Fungal immunomodulatory proteins (FIPs) are a group of low-molecular-weight (MW) proteins investigated as potential anti-tumor drugs. FIP-nha (from Nectria haematococca) contains two glycosylation sites at positions N5 and N39. In this study, the impact of glycosylation on the bioactivity and biochemical characteristics of FIP-nha (from Nectria haematococca) is described. Taken together, these findings indicate that glycosylation of FIP-nha impacts its thermostability and digestion resistance.

To study the impact of glycosylation on functionality of rFIP-nha, two single mutants (N5A and N39A) and one double mutant (N5+39A) were constructed to remove glycosylation sites. The SDS-PAGE results showed that the purified WT, N5A and N39A were partially glycosylated, while the N5+39A variant was indeed unglycosylated. However, we only managed to obtain crystals and solved the structures of WT, N39A and N5+39A. Unfortunately, none of the structures contained a density indicative of N-glycosylation. SLS and native-PAGE results suggested that rFIP-nha and its variants were all homogeneously tetrameric in the solution. The Tm values for WT, N5A, N39A and N5+39A were 82.2 °C, 81.4 °C, 80.7 °C and 80.1 °C, respectively. The stability of rFIP-nha during pepsin digestion was in this order: WT (T1/2 11.6 min) > N39A (T1/2 1.9 min) > N5A (T1/2 1.3 min) > N5+39A (T1/2 0.5 min). Double glycosylation significantly enhanced the pepsin resistance. Resistance to trypsin digestion is shown in Figure 6: N5A (T1/2 longer than 240 min) > WT (T1/2 89.3 min) > N5+39A (T1/2 13.9 min) > N39A (T1/2 8.1 min). Interestingly, 39N-glycosylation contributed to trypsin resistance, while 5N-glycosylation did not contribute to this resistance. Thus, both glycan chains appeared to be able to shield pepsin cleavage sites, possibly by steric hindrance, explaining the observed decrease in pepsin resistance in all mutants.

>GPLGSMATTNDSAVLFYIVASQKKLSFDYTPNWGRGSPNSYIDALTFPRVLTNKPYKYRVVKAGQDLGVRDSYSVQSDGSQKVNFLEYNAGRGIADTQTIQVYVVDPDNGNQYLVAQWKHHHHHH[4x]>IPNKRKPYKPCKNLVFYFHDILYNGKNAANATSAIVAAPEGVSLTKLAPQSHFGNIIVFDDPITLSHSLSSKQVGRAQGFYIYDTKNTYTSWLSFTFVLNSTHHQGTITFAGADPIVAKTRDISVTGGTGDFFMHRGIATITTDAFEGEAYFRLGVYIKFFECW[2x]

The entry point into presumed phenoxy radical-radical coupling to the 8–8′ lignan class involves one electron oxidation of the monolignol, e.g. coniferyl alcohol, which in the presence of a specific type of dirigent protein (DP; from the Latin dirigere, to guide or to align)2 (3), can undergo distinct forms of stereoselective coupling to afford either the (+)- or the (−)-antipode of pinoresinol (2a or 2b). Mechanistically, one electron oxidation (e.g. catalyzed by laccases, peroxidases) is envisaged to generate the corresponding coniferyl alcohol (1)-derived free radical intermediate (CA•), which then binds to the DPs. Bound substrate orientation subsequently occurs in such a way as to enable 8–8′ coupling at the si-si face with concomitant intramolecular cyclization to afford (+)-pinoresinol, such as in Forsythia intermedia, Thuja plicata, Schizandra chinensis, or pea (Pisum sativum), or alternatively re-re coupling to give the (−)-antipode as in Arabidopsis and flax (Linum usitatissimum). DPs are involved in lignan biosynthesis, whereas dirigent domains/sites have been implicated in lignin deposition.

In this investigation, determination of the x-ray crystal structure of the (+)-pinoresinol-forming DP PsDRR206 is reported. PsDRR206 structure was solved by molecular replacement and refined at 1.95 Å resolution. The asymmetric unit contains two independent molecules related by a noncrystallographic 2-fold rotation axis and connected by a single salt bridge between Glu169 and Arg173. The structure of the PsDRR206 monomer can be best described as an eight-stranded antiparallel β-meander forming a β-barrel. Analysis of the crystal symmetry shows that PsDRR206 forms a tightly packed trimer, with the trimer axis being orientated along the 3-fold axis of the H32 space group. Inspection of the trimer shows that the loop between the first two strands is involved in a domain-swapping event, wherein the loop does not simply reverse direction and become the second β-strand in the same monomer. Instead, it traverses the interface into the neighboring monomer, such that the N-terminal half of the first strand β2 is inserted into the second monomer next to its strand β2, adding a sixth strand to β-sheet 1. At the top of each barrel and slightly toward the outside of the trimer is a substantial pocket lined mostly with hydrophobic residues. Two polar residues, Asp40 and Arg141, conserved in all pinoresinol-forming DPs but not AOCs, are also located at either end of the pocket. In this regard, determination of the PsDRR206 three-dimensional structure, and its analysis suggests that the corresponding trimer has three identical substrate binding sites that are spatially distributed so that intermolecular coupling apparently cannot occur between two distinct substrate binding sites in the trimer model.2-{[(2S)-2-HYDROXY-3-(9-PHENANTHRYLOXY)PROPYL]AMINO}PROPANE-1,3-DIOL 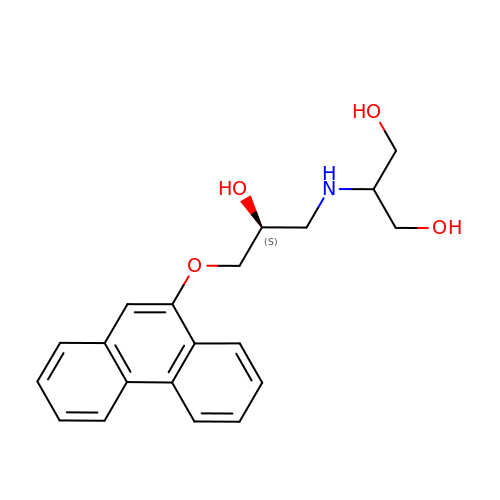| C20 H23 N O4 | WXMOCMHFWHZBSU-INIZCTEOSA-N> MSKAVNKKGLRPRKSDSILDHIKNKLDQEFLEDNENG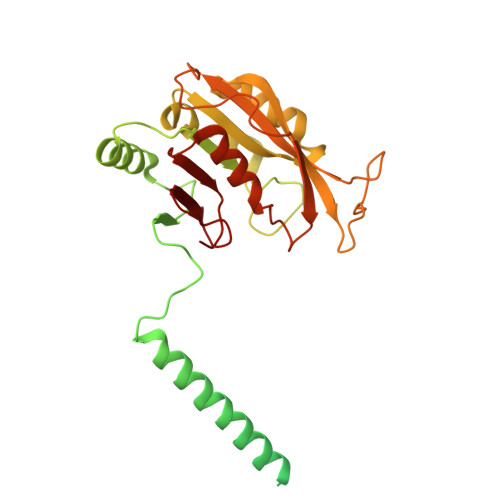EQSDEDYDQKSLNKAKKPYKKRQTQNGSELVISQQKTKAKASANNKKSAKNSQKLDEEEKIVEEEDLSPQKNGAVSEDDQQQEASTQEDDYLDRLPKSKKGLQGLLQDIEKRILHYKQLFFKEQNEIANGKRSMVPDNSIPICSDVTKLNFQALIDAQMRHAGKMFDVIMMDPPWQLSSSQPSRGVAIAYDSLSDEKIQNMPIQSLQQDGFIFVWAINAKYRVTIKMIENWGYKLVDEITWVKKTVNGKIAKGHGFYLQHAKESCLIGVKGDVDNGRFKKNIASDVIFSERRGQSQKPEEIYQYINQLCPNGNYLEIFARRNNLHDNWVSIGNEL>[6x]MTRRYLKYYIFVTLLFFVQVINNVLCAPDNKQEQGKYLNRTINILNAGKNIAKSYGHNKLKPIHILSALAKSDYGSTLFKENNVNAANLKEYIDIALEQTRAGAPLDNKSKIVNSAEVKETLALAEAAANKYKSPKVDVEHLLSGLSNDELVNEIFNEVYLTDEAIKAILKRKFEKTKKDKDGKTGTLYIEQFGSNMNEKVRNGKLQGIYGRDEEIRAIIESLLRYNKNSPVLVGNPGTGKTTIVEGLVYRIEKGDVPKELQGY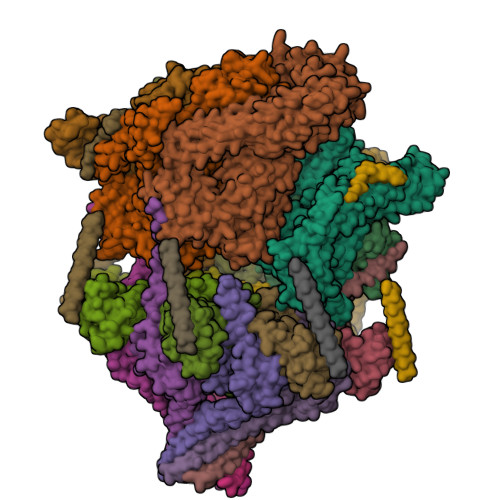TVISLNFRKFTSGTSYRGEFETRMKNIIKELKNKKNKIILFVDEIHLLLGAGKAEGGTDAANLLKPVLSKGEIKLIGATTIAEYRKFIESCSAFERRFEKILVEPPSVDMTVKILRSLKSKYENFYGINITDKALVAAAKISDRFIKDRYLPDKAIDLLNKACSFLQVQLSGKPRIIDVTERDIERLSYEISTLEKDVDKVSKKKYNKLIKEFEEKKEQLKKYYEEYVITGERLKRKKEIEKKLNDLKELTQNYVYSNKEPPIELQNSLKEAQQKYLELYKETVAYVEAKTHNAMNVDAVYQEHVSYIYLRDSGMPLGSLSFESSKGALKLYNSLSKSIIGNEDIIKSLSDAVVKAATGMKDPEKPIGTFLFLGPTGVGKTELAKTLAIELFNSKDNLIRVNMSEFTEAHSVSKITGSPPGYVGFSDSGQLTEAVREKPHSVVLFDELEKAHADVFKVLLQILGDGYINDNHRRNIDFSNTIIIMTSNLGAELFKKKLFFDADNSGTPEYKRVMEDVRLSLIKKCKKVFKPEFVNRIDKIGVFEPLNKKNLHKIVALRFKKLEKRLEEKNIQVSVSEKAIDYIIDQSYDPELGARPTLIFIESVIMTKFAIMYLKKELVDDMDVFVDYNSKAKNLVINLSKTPRDYKDDDDKDYKDDDDKDYKDDDDK;>MKVSYIFSFFLLFFVYKNTNTVVCDNGYGDLAATSALTTVIKDPISLTIKDIYEHGVKNPFTKIIHKLKKFIRYRKVLRWSRMWWVLLVREIVGDNTIEKKTEKALREIWDQCTIAVYNNTLNAVESKPLLFLHGILNECRNNFATKLRQDPSLIVAKIDQIIKSQIYRFWVSEPYLKIGRSHTLYTHITPDAVPQLPKECTLKHLSSYMEEKLKSMESKKNIESGKYEFDVDSSETDSTKDDGKPDDDDDDDDNFDDDDNFDDDTVEEEDASGDLFKNEKKDENKE[7x]> GGAUCUUCGGGGCAGGGUGAAAUUCCCGACCGGUGGUAUAGUCCACGAAAGUAUUUGCUUUGAUUUGGUGAAAUUCCAAAACCGACAGUAGAGUCUGGAUGAGAGAAGAUUC

The flavin mononucleotide (FMN) riboswitch, or RFN element, is a widespread and highly conserved RNA structural element present in the eubacterial operons of genes involved in riboflavin biosynthesis and transport (Gelfand et al., 1999, Gusarov et al., 1997, Vitreschak et al., 2002). In response to intracellular concentrations of FMN, a derivative of vitamin B2, the FMN riboswitch in most bacteria follows a mechanism of transcription attenuation, whereby ligand binding to the aptamer domain leads to the formation of an intrinsic terminator hairpin followed by a uridine track in the downstream expression platform (Wickiser et al., 2005, Winkler et al., 2002). The FMN riboswitch aptamer from F. nucleatum exhibits a “butterfly-like” fold, whose six helical domains form nearly symmetrical “wings” with a central junction area that includes the FMN binding site (Serganov et al., 2009, Vicens et al., 2011). Ligand-induced stabilization of the aptamer’s P1 helix results in the formation of an intrinsic terminator stem in the expression platform.

We have identified a ligand-free structure of the aptamer that provides further insight into the conformational switching mechanism that enables genetic control by this riboswitch. In the absence of FMN, the helical structures of P3 and P4 are aligned, the stacking continuity of which is facilitated by junction residues G47, A48, and U61. This results in misalignment of P1 and P6, destabilizing P1, and liberating the switching sequence that includes J1/2. Specifically, P6 residues (A85, G98, A99), located on the isoalloxazine-side of the FMN binding pocket, remain relatively fixed, whereas junction residues G47, A48, A49 bridge and conduct base stacking between helices P3 and P4. This is further stabilized by a non-Watson-Crick base pair between U61 and A48. The positions of the guanine residues (G10, G11, G32, G62, G84) that coordinate the FMN phosphate moiety are relatively unchanged. This is due, in part, to a sulfate ion that mimics the FMN phosphate with a similar coordination sphere. Several other crystal forms were obtained under conditions absent of tetrahedral anions. However, all such crystals diffracted very poorly (<10 Å resolution), most likely owing to increased flexibility of J1/2 and instability of P1. Despite involving minimal changes in or near the binding pocket, FMN binding switches the direction of productive base stacking, not only within the junction, but more importantly across the junction, from collinearity of P3/P4 (apo) to collinearity of P1/P6 (holo).> MLKQVEIFTDGSCLGNPGPGGYGAILRYRGREKTFSAGYTRTTNNRMELMAAIVALEALKEHCEVILSTDSQYVRQGITQWIHNWKKRGWKTADKK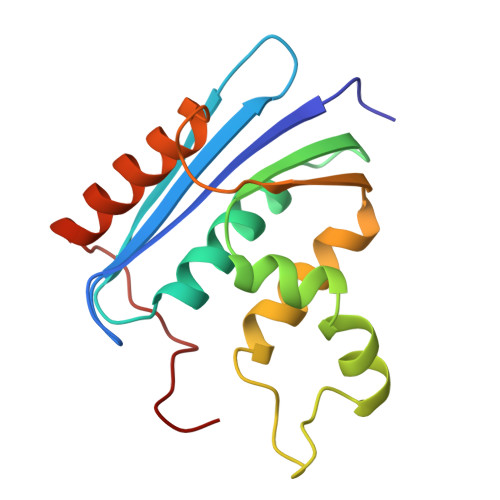PVKNVDLWQRLDAALGQHQIKWEWVKGHAGHPENERCHELARAAAMNPTLEDTGYQVEV4-(3-METHYLPHENYL)-1H-1,2,3-TRIAZOLE | C9 H9 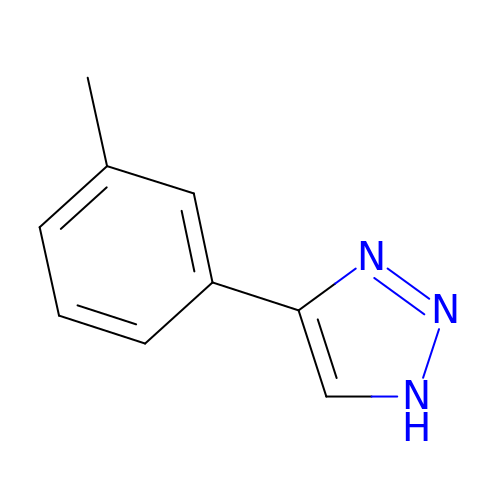N3 | XQHCBHNLRWLGQS-UHFFFAOYSA-N>[2x]SVPGRKFIAVKAHSPQGEGEIPLHRGEAVKVLSIGEGGFWEGTVKGRTGWFPADCV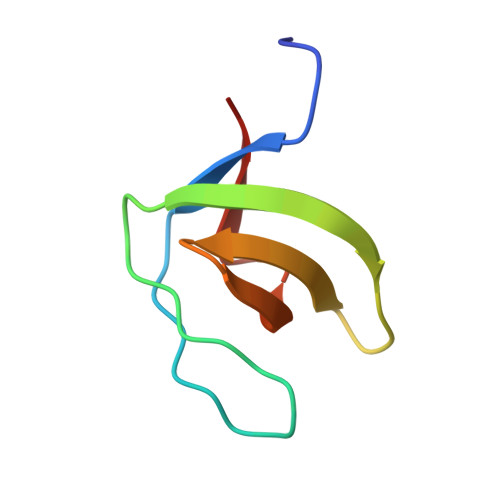EEVQ>MKLYYSPGACSLSPHIALREAGLNFELVQVDLASKKTASGQDYLEVNPAGYVPCLQLDDGRTLTEGPAIVQYVADQVPGKQLAPANGSFERYHLQQWLNFISSELHKSFSPLFNPASSDEWKNAVRQSLNTRLGQVARQLEHAPYLLGDQLSVADIY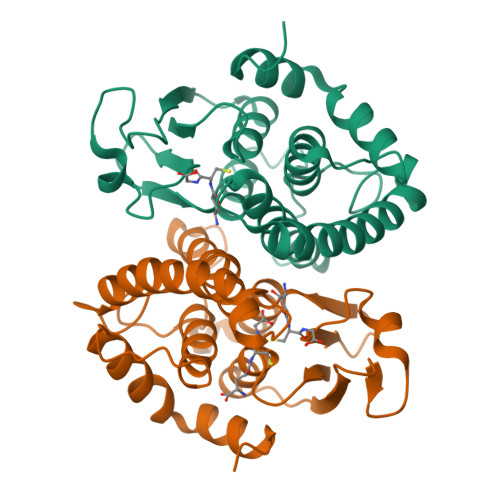LFVVLGWSAYVNIDLSPWPSLQAFQGRVGGREAVQSALRAEGLIK[6x]12-(diethylamino)-2,2-bis(fluoranyl)-4,5-dimethyl-5-aza-3-azonia-2-boranuidatricyclo[7.4.0.0^{3,7}]trideca-1(13),3,7,9,11-pentaen-6-one | C16 H20 B F2 N3 O | 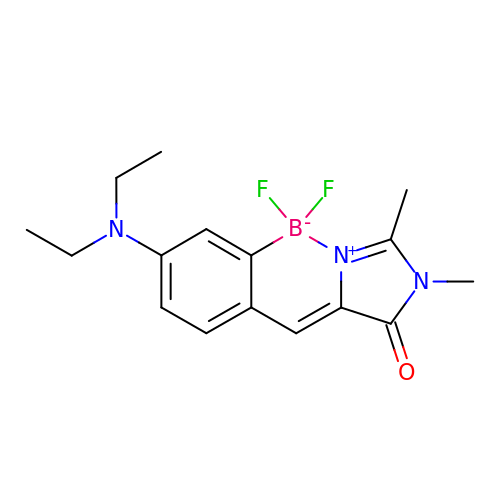OOEJBECJAKZKRT-UHFFFAOYSA-N1-phenyl-5-(trifluoromethyl)pyrazole-4-carboxylic 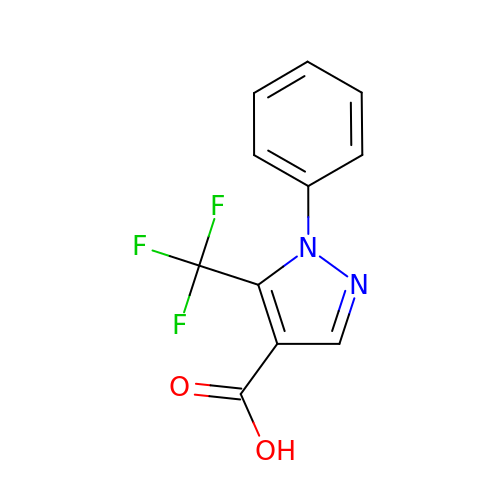acid | C11 H7 F3 N2 O2 | SMPJBTIFNUUWGQ-UHFFFAOYSA-N> VLDINDNEPVFTQDVFVGSVEELSAAHTLVMKINATDADEPNTLNSKISYRIVSLEPAYPPVFYLNKDTGEIYTTSVTLDREEHSSYTLTVEARDGNGEVTDKPVKQAQVQIRILDVNDNIPVVENKVLEGMVEENQVNVEVTRIKVFDADEIGSDNWLANFTFASGNEGGYFHIETDAQTNEGIVTLIKEVDYEEMKNLDFSVIVANKAAFHKSIRSKYK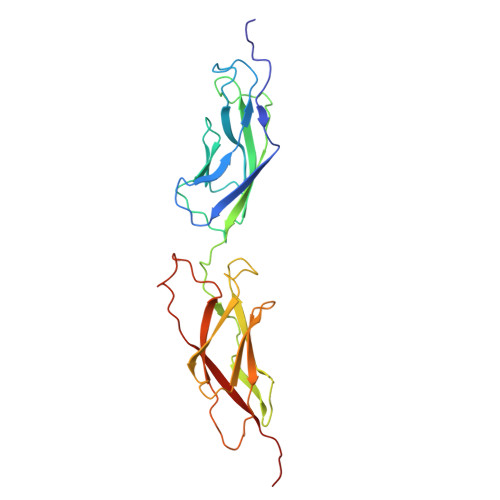PTPIPIKVKVKNVKEGI> SSSASGGSKIPNTSLFVPLTVKPQGPSADGDVGAELTRPLDKNEVKKVLDKFYKRKEIQKLGADYGLDARLFHQAFISFRNYIMQSHSLDVDIHIVLN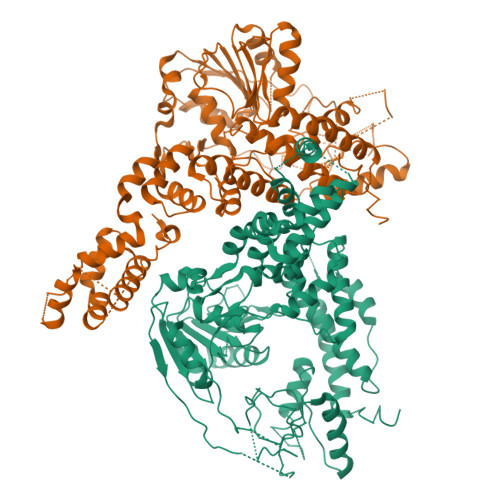DICFGAAHADDLFPFFLRHAKQIFPVLDCKDDLRKISDLRIPPNWYPDARAMQRKIIFHSGPTNSGKTYHAIQKYFSAKSGVYCGPLKLLAHEIFEKSNAAGVPCDLVTGEERVTVQPNGKQASHVSCTVEMCSVTTPYEVAVIDEIQMIRDPARGWAWTRALLGLCAEEVHLCGEPAAIDLVMELMYTTGEEVEVRDYKRLTPISVLDHALESLDNLRPGDCIVCFSKNDIYSVSRQIEIRGLESAVIYGSLPPGTKLAQAKKFNDPNDPCKILVATDAIGMGLNLSIRRIIFYSLIKPSINEKGERELEPITTSQALQIAGRAGRFSSRFKEGEVTTMNHEDLSLLKEILKRPVDPIRAAGLHPTAEQIEMFAYHLPDATLSNLIDIFVDFSQVDGQYFVCNMDDFKFSAELIQHIPLSLRVRYVFCTAPINKKQPFVCSSLLQFARQYSRNEPLTFAWLRRYIKWPLLPPKNIKDLMDLEAVHDVLDLYLWLSYRFMDMFPDASLIRDLQKELDGIIQDGVHNITKLIKMSETHKLLNLEGFPSGSQSRLSGTLKSQARRTRGTKALGSKATE> GMHTQEALFVRLALDAWNTQSSRTDKLIQSLSNEALAVETAPGRNSGTYLLGHLTAVHDAMLPLLELGDTLYPQLAPVFIQNPDKSGLEKPEINDLRLYWSLVQERLANQFNQLQPADWFNKHAAISREDFLKEPHRNKLSVLINRTNHM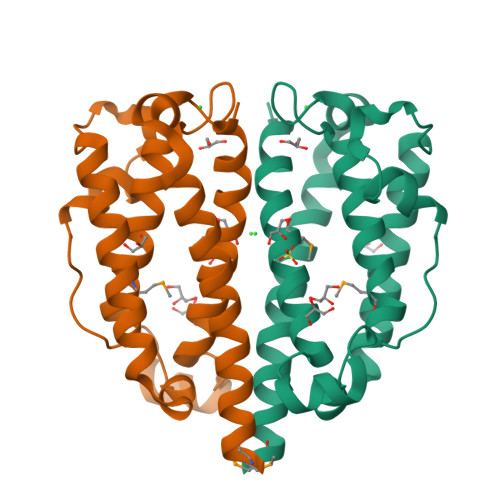AYHLGQLAYLKK4-[2-({methyl[(pyridin-3-yl)methyl]amino}methyl)-1,3-thiazol-4-yl]piperidin-4-ol 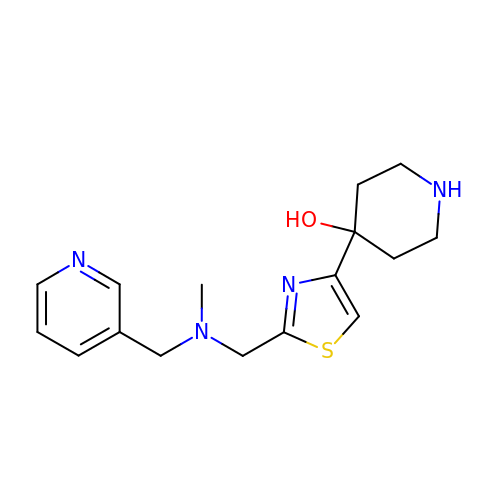| C16 H22 N4 O S | QKMHFIHZICPGSU-UHFFFAOYSA-N> AGASRQRKLEALIRDPRSPINVESLLDGLNSLVLDLDFPALRKNKNIDNFLNRYEKIVKKIRGLQMKAEDYDVVKVIGRGAFGEVQLVRHKASQKVYAMKLLSKFEMIKRSDSAFFWEERDIMAFANSPWVVQLFYAFQDDRYLYMVMEYMPGGDLVNLMSNYDVPEKWAKFYTAEVVLALDAIHSMGLIHRDVKPDNMLLDKHGHLKLADFGTCMKMDETGMVHCDTAVGTPDYISPEVLKSQGGDGFYGRECDWWSVGVFLYEMLVGDTPFYADSLVGTYSKIMDHKNSLCFPEDAEISKHAKNLICAFLTDREVRLGRNGVEEIRQHPFFKNDQWHWDNIRE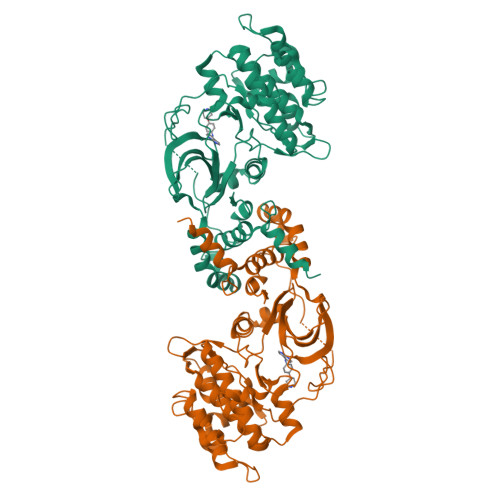TAAPVVPELSSDIDSSNFDDIEDDKGDVETFPIPKAFVGNQLPFIGFTYYR>HHHHHHGCMSGRKPIIGVMGPGKADTAENQLVMANELGKQIATHGWILLTGGRSLGVMHEAMKGAKEAGGTTIGVLPGPDTSEISDAVDI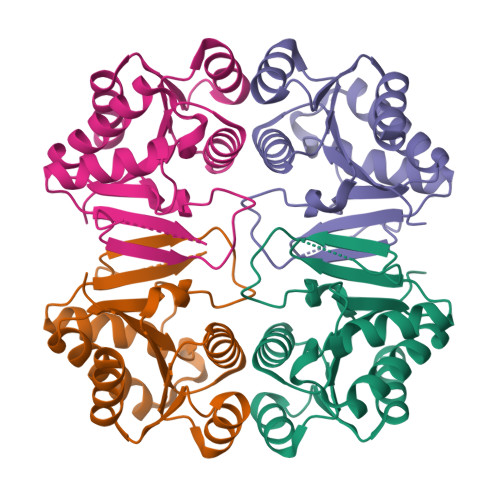PIVTGLGSARDNINALSSNVLVAVGMGPGTAAEVALALKAKKPVVLLGTQPEAEKFFTSLDAGLVHVAADVAGAIAAVKQLLAKLN[2x]> MEPHSLRYNLTVLIWDGSVQSGFLTEVHLDGQPFLRCDRQKCRAKPQGQWAEDVLGNKTWDRETRDLTGNGKDLRMTLAHIKDQKEGLHSLQEIRVCEIHEDNSTRSSIHFYYDGELFLSNNLETKEWTMPQSSRAQTLAMNVRNFWKEDAM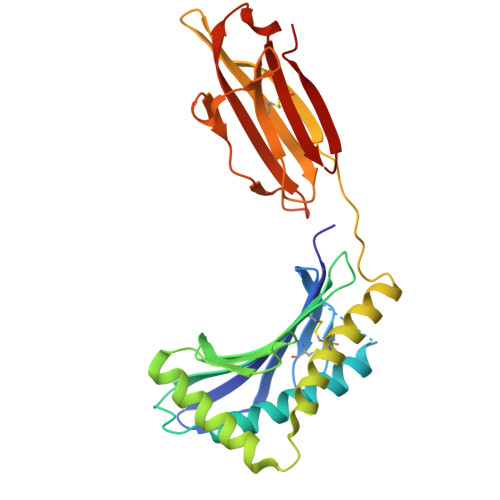KTKTHWHAMHADCLQELRRYLKSGVVLRRTVPPMVNVTRSEASEGNITVTCRASGFYPWNITLSWRQDGVSLSHDTQQWGDVLPDGNGTYQTWVATRICQGEEQRFTCYMEHSGNHSTHPVPS> VPPGGEPLYTEQDLAVNGREGFPNYRIPALTVTPDGDLLASYDGRPTGIDAPGPNSILQRRSTDGGRTWGEQQVVSAGQTTAPIKGFSDPSYLVDRETGTIFNFHVYSQRQGFAGSRPGTDPADPNVLHANVATSTDGGLTWSHRTITADITPDPGWRSRFAASGEGIQLRYGPHAGRLIQQYTIINAAGAFQAVSVYSDDHGRTWRAGEAVGVGMDENKTVELSDGRVLLNSRDSARSGYRKVAVSTDGGHSYGPVTIDRDLPDPTNNASIIRAFPDAPAGSARAKVLLFSNAASQTSRSQGTIRMSCDDGQTWPVSKVFQPGSMSYSTLTALPDGTYGLLYEPGTGIRYANFNLAWLGGICAPFTIPDVALEPGQQVTVPVAVTNQSGIAVPKPSLQLDASPDWQVQGSVEPLMPGRQAKGQVTITVPAGTTPGRYRVG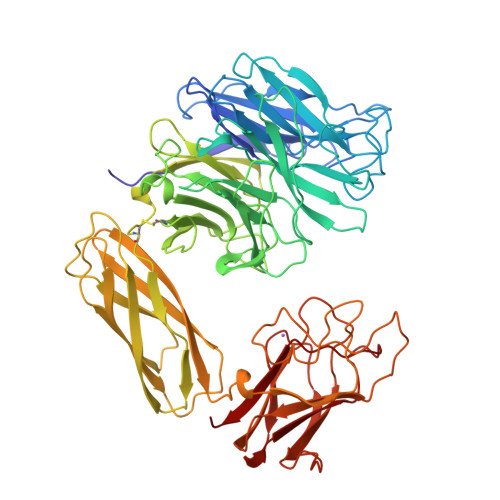ATLRTSAGNASTTFTVTVGLLDQARMSIADVDSEETAREDGRASNVIDGNPSTFWHTEWSRADAPGYPHRISLDLGGTHTISGLQYTRRQNSANEQVADYEIYTSLNGTTWDGPVASGRFTTSLAPQRAVFPARDARYIRLVALSEQTGHKYAAVAELEVEGQR>WGNLGHETVAYIAQSFVASSTESFCQNILGDDSTSYLANVATWADTYKYTDAGEFSKPYHFIDAQDNPPQSCGVDYDRDCGSAGCSISAIQNYTNILLESPNGSEALNALKFVVHIIGDIHQPLHDENLEAGGNGIDVTYDGETTNLHHIWDTNMPEEAAGGYSLSVAKTYADLLTERIKTGTYSSKKDSWTDGIDIKDPVSTSMIWAADANTYVCSTVLDDGLAYINSTDLSGEYYDKSQPVFEELIAKAGYRLAAWLDLI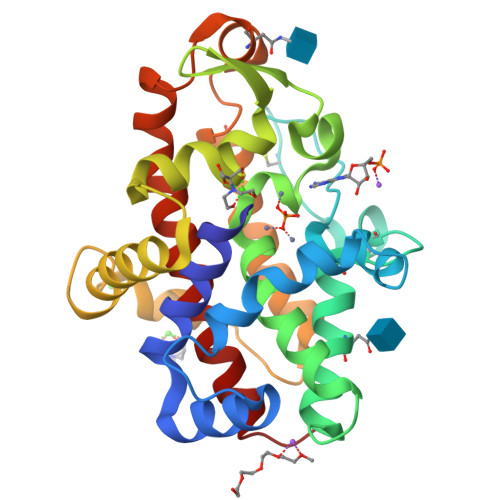ASQPS[2x]>[2x]SNPRLTKVLDEMSKKPCVNINEIRKMIRNFQPQFIQPRNGNRPNAQPRTVDSFEWVVRIQSTVETQLLGATNTVPQQTLNLDISFTDDSTTITPASIPGSISMLDNSRHIPAIQSMIQNFKARYLGSLQDTAQLQSPQYPQLLAYLFGQLIAIKDRLDLFRPSNPLSLADALFGFTLAQNARPRYDDHRHAKACQGPLVIPAA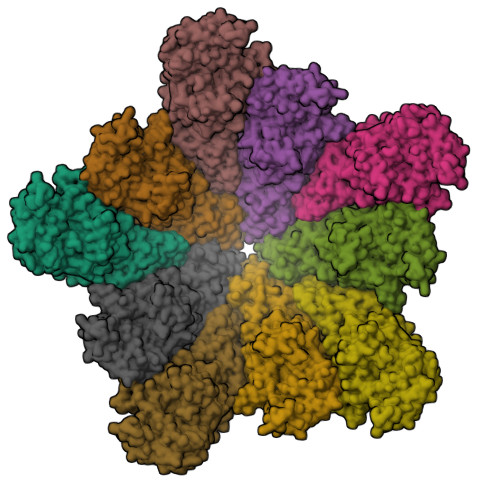TNSDCGPCGFVQINANQGLTLPLGACLFVNPETVNDQSFQDFLWLIFATHHRMPNQMQNNWPFSLNIVSTCAAPGRQAPHAGELTDERVRLALDTGHRILLSMFNDDEETLRYYQRKGIETMFRPCCFYTEGGLLRKATRYVSMVPLNGLYYYNGATSYVVSPIHTDAHPGITAAIESFVDIMVLQAVFSFSGPKVVAAKVNASQIDAAMVFGPAVAEGDGFVYDPLRPAPPLSAFYTEFIHRPAEQRIFQMAMSQIYGSHAPLIIANVINSIHNCKTKIVNNKLRATFVRRPPGAPHLKADTAIINRFHDPELAYALGILADGIAPLDGSHEYNVLDELDYLFNGGDIRNCFGLNALNTRGLGQIVHIRPKREPGKRPRRGFYTTLDGQVHPVTQDAPLDEIYHWRDHGNLTRPYSCHILDSQGLEFADVSNGRSRGKILVVVNSPLKTCAAYQGPSFAPK> SNADSLPERIDLFVSLFDYNSATTSYDIRSIQTDFPTRLLTPDSMLPQTSEYPLKDIQLLYKLAQSCTGKLPLSPLITEPLVFTRSLCKGSSLSPRWFARSGLIHPGGGTYAFRYAEKYPAQFANLLPYMHIQERPNAAEGTLLYHLQNMGEDAINA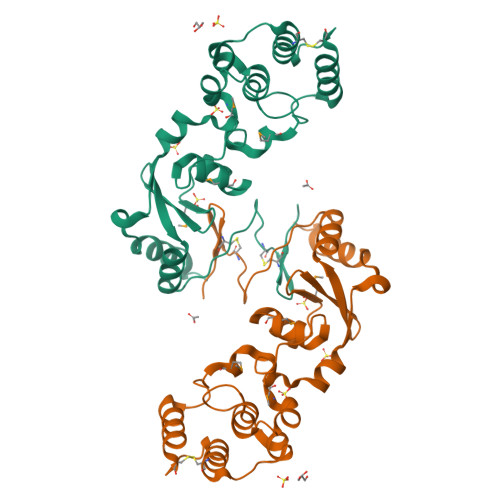LVSGASMFGSGSDLWLRKGDIYYLFNEETWLTNANKAGLSYSLLSADNTCFIQRGNICWDVEDHS>[2x]MVEHDKSGSKRQELRSNMRNLITLNKGKFKPTASTAEGDEDDLSFTLLDSVFDTLSDSITCVLGSTDIGAIEVQQFMKDGSRNVLASFNIQTFDDKLLSFVHFADINQLVFVFEQGDIITATYDPVSLDPAETLIEIMGTIDNGIAAAQWSYDEETLAMVTKDRNVVVLSKLFEPISEYHLEVDDLKISKHVTVGWGKKETQFRGKGARAMEREALASLKASGLVGNQLRDPTMPYMVDTGDVTALDSHEITISWRGDCDYFAVSSVEEVPDEDDETKSIKRRAFRVFSREGQLDSASEPVTGMEHQLSWKPQGSLIASIQRKTDLGEEDSVDVIFFERNGLRHGEFDTRLPLDEKVESVCWNSNSEALAVVLANRIQLWTSKNYHWYLKQELYASDISYVKWHPEKDFTLMFSDAGFINIVDFAYKMAQGPTLEPFDNGTSLVVDGRTVNITPLALANVPPPMYYRDFETPGNVLDVACSFSNEIYAAINKDVLIFAAVPSIEEMKKGKHPSIVCEFPKSEFTSEVDSLRQVAFINDSIVGVLLDTDNLSRIALLDIQDITQPTLITIVEVYDKIVLLRSDFDYNHLVYETRDGTVCQLDAEGQLMEITKFPQLVRDFRVKRVHNTSAEDDDNWSAESSELVAFGITNNGKLFANQVLLASAVTSLEITDSFLLFTTAQHNLQFVHLNSTDFKPLPLVEEGVEDERVRAIERGSILVSVIPSKSSVVLQATRGNLETIYPRIMVLAEVRKNIMAKRYKEAFIVCRTHRINLDILHDYAPELFIENLEVFINQIGRVDYLNLFISCLSEDDVTKTKYKETLYSGISKSFGMEPAPLTEMQIYMKKKMFDPKTSKVNKICDAVLNVLLSNPEYKKKYLQTIITAYASQNPQNLSAALKLISELENSEEKDSCVTYLCFLQDVNVVYKSALSLYDVSLALLVAQKSQMDPREYLPFLQELQDNEPLRRKFLIDDYLGNYEKALEHLSEIDKDGNVSEEVIDYVESHDLYKHGLALYRYDSEKQNVIYNIYAKHLSSNQMYTDAAVAYEMLGKLKEAMGAYQSAKRWREAMSIAVQKFPEEVESVAEELISSLTFEHRYVDAADIQLEYLDNVKEAVALYCKAYRYDIASLVAIKAKKDELLEEVVDPGLGEGFGIIAELLADCKGQINSQLRRLRELRAKKEENPYAFYGQETEQADDVSVAPSETSTQESFFTRYTGKTGGTAKTGASRRTAKNKRREERKRARGKKGTIYEEEYLVQSVGRLIERLNQTKPDAVRVVEGLCRRNMREQAHQIQKNFVEVLDLLKANVKEIYSISEKDRERVNENGEVYYIPEIPVPEIHDFPKSHIVDF;> MVECITPEAIFIGANKQTQVSDIHKVKKIVAFGAGKTIALWDPIEPNNKGVYATLKGHEAEVTCVRFVPDSDFMVSASEDHHVKIWKFTDYSHLQCIQTIQHYSKTIVALSALPSLISVGCADGTISIWRQNIQNDEFGLAHEFTIKKGFFYPLCLSLSKVEEKKYLLAIGGTNVNVFIASFILSDSGIEKCRVVAELEGHEDWVKSLAFRHQETPGDYLLCSGSQDRYIRLWRIRINDLIDDSEEDSKKLTLLSNKQYKFQIDDELRVGINFEALIMGHDDWISSLQWHESRLQLLAATADTSLMVWEPDETSGIWVCSLRLGEMSSKGASTATGSSGGFWSCLWFTHERMDFFLTNGKTGSWRMWATKDNIICDQRLGISGATKDVTDIAWSPSGEYLLATSLDQTTRLFAPWIYDASGRKREIATWHEFSRPQIHGYDMICVETVTDTRFVSGGDEKILRSFDLPKGVAGMLQKFVGIQFEEKSEMPDSATVPVLGLSNKAGEDDANEDDEEEEGGNKETPDITDPLSLLECPPMEDQLQRHLLWPEVEKLYGHGFEITCLDISPDQKLIASACRSNNVQNAVIRIFSTENWLEIKPALPFHSLTITRLKFSKDGKFLLSVCRDRKWALWERNMEDNTFELRFKNEKPHTRIIWDADWAPLEFGNVFVTASRDKTVKVWRHQKEPADDYVLEASIKHTKAVTAISIHDSMIREKILISVGLENGEIYLYSYTLGKFELITQLNEDITPADKITRLRWSHLKRNGKLFLGVGSSDLSTRIYSLAYE;> MARHGKGPKTNKKKLAPEKERFIQCCADITLELTDSLTSGTTREINLNGLITKYSKKYKLKQQPRLTDIINSIPDQYKKYLLPKLKAKPVRTASGIAVVAVMCKPHRCPHIAYTGNICVYCPGGPDSDFEYSTQSYTGYEPTSMRAIRARYDPYEQARGRVEQLKQLGHSIDKVEYVLMGGTFMSLPKEYREDFIVKLHNALSGFNGNDIDEAILYSQQSLTKCVGITIETRPDYCTQTHLDDMLKYGCTRLEIGVQSLYEDVARDTNRGHTVRSVCETFAVSKDAGYKVVSHMMPDLPNVGMERDIEQFKEYFENPDFRTDGLKIYPTLVIRGTGLYELWKTGRYKSYSANALVDLVARILALVPPWTRIYRVQRDIPMPLVTSGVDNGNLRELALARMKDLGTTCRDVRTREVGIQEVHHKVQPDQVELIRRDYYANGGWETFLSYEDPKKDILIGLLRLRKASKKYTYRKEFTSQRTSIVRELHVYGSVVPLHSRDPRKFQHQGFGTLLMEEAERIAKEEHGSEKISVISGVGVRNYYGKLGYELDGPYMSKRI

In eukaryotes, wobble uridines are modified by Elongator, a large and highly conserved macromolecular complex. Elongator consists of two subcomplexes, namely Elp123 containing the enzymatically active Elp3 subunit and the associated Elp456 hetero-hexamer. The Elongator complex harbors two copies of each of its six subunits, namely Elongator proteins 1–6 (Elp1–Elp6). Decreased levels of wobble uridine modifications lead to ribosome pausing, incorrect protein folding and consequently trigger intracellular protein aggregation and proteotoxic stress.

Meanwhile, we also collected a dataset for ScElp123 in complex with yeast tRNA AlaUGC and obtained a reconstruction at an improved resolution of 3.96 Å. This new tRNA-bound structure of ScElp123 allowed us to build a more reliable atomic model of the tRNA-bound complex, which facilitated the structural comparison of individual regions in ScElp123 and MmElp123. Although we did not supplement the sample with SAM before vitrification, we identified a bound 5′-dA molecule in the yeast active site next to the cluster. Gln257 contacts one of the hydroxyl groups in 5′-dA and positions the radical carrying methyl group in close proximity to Tyr136 and Tyr327, which both are positioned in a similar distance to the base of U34 and to the methyl group of 5′-dA. Furthermore, we observed that the density of Tyr136 connects to the one of U34, suggesting direct interaction. This tyrosine possibly pulls the uridine closer to the iron-sulfur cluster and the 5′-dA molecule. As for the fourth iron atom of the cluster, it is not coordinated by any cysteine residue but it is bordered by an additional, adjacent density, which most likely can be attributed to bound methionine. Second, the ScElp123 in complex with tRNA harbors the SAM cleavage products, namely 5′-dA and methionine, in its catalytic site.> SMTRIIGGVAGGRRIAVPPRGTR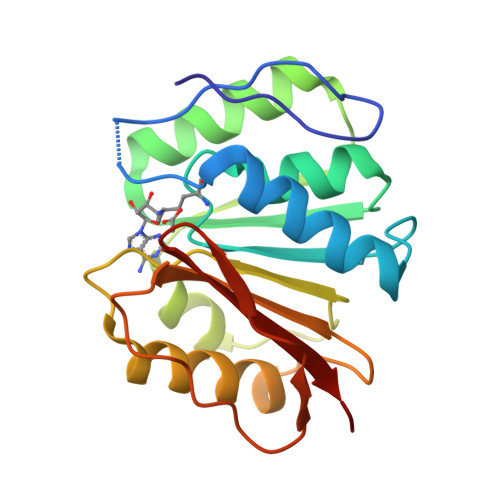PTTDRVRESLFNIVTARRDLTGLAVLDLYAGSGALGLEALSRGAASVLFVESDQRSAAVIARNIEALGLSGATLRRGAVAAVVAAGTTSPVDLVLADPPYNVDSADVDAILAALGTNGWTREGTVAVVERATTCAPLTWPEGWRRWPQRVYGDTRLELAERLFANV>MEGLNLVATALAVGLGAIGPGVGIGIIVSGAVQAIGRNPEIENRVVTYMFIGIAFTEALAIFGLVIAFLIGFGVLQ[10x];>MSTRTRNILIIVGALIISIASRFFLYTGPPHVEVAAEVIFDGIPGFPITNSFVVAIIIDIFVIALAVAATRNLQMVPRGLQNVMEFILESLYNLFRNINAKYVATAFPLVATIFLFVLFGNWFGLLPGVGSIGVCHEKKEEHAVVDERLALAAPAAPLSSVAAAEGEEIHDTCAAQGKKLVPLFRAPAADLNFTFAIAVISFVFIEYWGFRALGPGYLKKFFNTNGIMSFVGIIEFISELVKPFALAFRLFG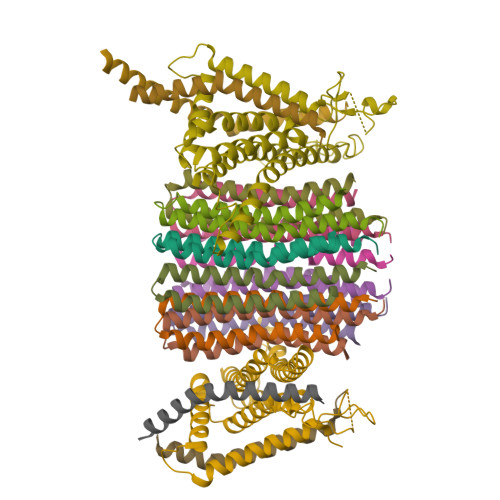NIFAGEVLLVVMAFLVPLLLPLPFYGFEVFVGFIQALIFALLTYAFLNIAVTGHDEEHAH[2x];>[4x]MEALGINPTLFIAQLINFLLLIFILRALLYRPVMNLLNERTRRIEESVRDAEKVREQLANARRDYEAEIARARQEAAKIVAQAQERAKQQEAEIIAQARREAERLKEEARAQAEQERIRMLSEAKSQIADLVTLTASRVLGAELQARGHDALIAESLAALDRRN>[2x]GSHMASELNEHRATLFNKNVPSRAVKRVTAITKVEREAVLVCELPSFDVTDVEFDLFRARESTDKPLDVAAAIAYRLLLGSGLPQKFGCSDEVLLNFILQCRKKYRNVPYHNFYHVVDVCQTIHTFLYRGNVYEKLTELECFVLLITA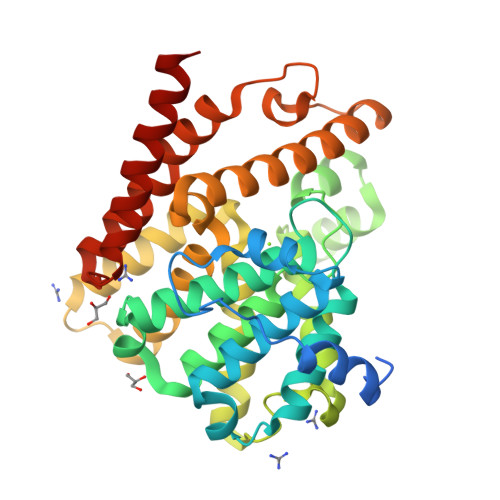LVHDLDHMGLNNSFYLKTESPLGILSSASGNTSVLEVHHCNLAVEILSDPESDVFDGLEGAERTLAFRSMIDCVLATDMAKHGSALEAFLASAADQSSDEAAFHRMTMEIILKAGDISNVTKPFDISRQWAMAVTEEFYRQGDMEKERGVEVLPMFDRSKNMELAKGQIGFIDFVAAPFFQKIVDACLQGMQWTVDRIKSNRAQWERVLETR> SAQTIEATSVKQLADAGVRVGDTLRISG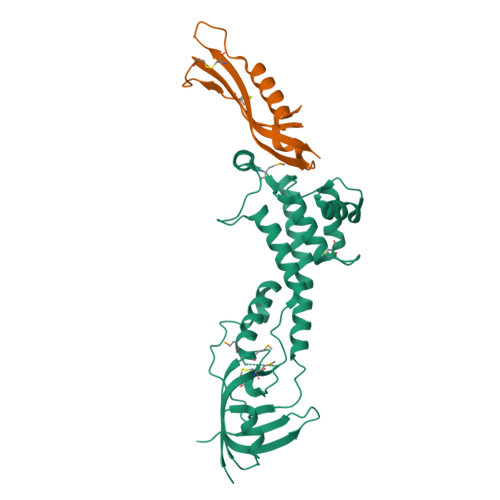TGMCNIRTSGTWSAKTNSPFLPFDCSQIIWNDARSLPLPESELVNKATALTEAVNRQLHPKPEDESRVSASLRSAIQKSGMVLLDDFGDIVLKTADLCSAKDDCVRLKNALVNLGNSKDWDALVKRANAGKLDGVNVLLRPVSAESLDNLVATSTAPFITHETARAAQSLNSPAPGGFLIVSDEGSDFVDQPWPSASLYDYPPQEQWNAFQKLAQMLMHTPFNAEGIVTKIFTDANGTQHIGLHPIP;> RATPVRIYTNAEELVGKPFRDLGEVSGDSCQASNQDSPPSIPTARKRMQINASKMKANAVLLHSCEVTSGTPGCYRQAVCIGSALNIT> GLGQMLESMIDNTVSSTVGAATSRDALPNTEASGPTHSKEIPALTAVETGATNPLVPSDTVQTRHVVQHRSRSESSIESFFARGACVTIMTVDNPASTTNKDK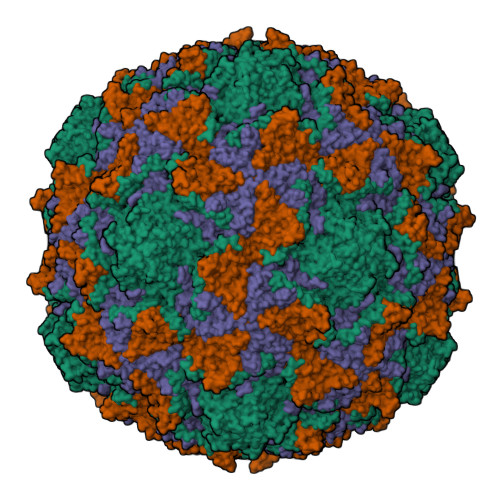LFAVWKITYKDTVQLRRKLEFFTYSRFDMELTFVVTANFTETNNGHALNQVYQIMYVPPGAPVPEKWDDYTWQTSSNPSIFYTYGTAPARISVPYVGISNAYSHFYDGFSKVPLKDQSAALGDSLYGAASLNDFGILAVRVVNDHNPTKVTSKIRVYLKPKHIRVWCPRPPRAVAYYGPGVDYKDGTLTPLSTKDLTTY;> SPNIEACGYSDRVLQLTLGNSTITTQEAANSVVAYGRWPEYLRDSEANPVDQPTEPDVAACRFYTLDTVSWTKESRGWWWKLPDALRDMGLFGQNMYYHYLGRSGYTVHVQCNASKFHQGALGVFAVPEMCLAGDSNTTTMHTSYQNANPGEKGGTFTGTFTPDNNQTSPARRFCPVDYLLGNGTLLGNAFVFPHQIINLRTNNCATLVLPYVNSLSIDSMVKHNNWGIAILPLAPLNFASESSPEIPITLTIAPMCCEFNGLRNITLPRLQ;> GLPVMNTPGSNQYLTADNFQSPCALPEFDVTPPIDIPGEVKNMMELAEIDTMIPFDLSATKKNTMEMYRVRLSDKPHTDDPILCLSLSPASDPRLSHTMLGEILNYYTHWAGSLKFTFLFCGSMMATGKLLVSYAPPGADPPKKRKEAMLGTHVIWDIGLQSSCTMVVPWISNTTYRQTIDDSFTEGGYISVFYQTRIVVPLSTPREMDILGFVSACNDFSVRLLRDTTHIEQKALAQ;> GAQVSSQKVGAHENSNRAYGGSTINYTTINYYRDSASNAASKQDFSQDPSKFTEPIKDVLIKTAPMLN Saposins A, B, C and D comprise a family of small, non-enzymatic lipid-transfer proteins that are essential for the activation of GSL catabolism; genetic defects in saposin function cause specific forms of lysosomal storage diseases. Each saposin shows functional specificity for the activation of certain catabolic reactions: saposin A (SapA) activates the hydrolysis of β-d-galactocerebroside to ceramide and galactose by the enzyme β-galactocerebrosidase (GALC; EC 3.2.1.46; Morimoto et al., 1989; Harzer et al., 1997). Whilst they share less than 35% sequence identity, they all adopt a common fold consisting of four amphipathic α-helices organized into two ‘fingers’. SapA is known to bind lipids and detergents in a pH-dependent manner; this is accompanied by a striking transition from a ‘closed’ to an ‘open’ conformation.

However, previous structures were determined at non-lysosomal pH. This work describes a 1.8 Å resolution X-ray crystal structure determined at the physiologically relevant lysosomal pH 4.8. In the absence of lipid or detergent at pH 4.8, SapA is observeed to adopt a conformation closely resembling the previously determined ‘closed’ conformation, showing that pH alone is not sufficient for the transition to the ‘open’ conformation. The asymmetric unit contains two molecules of SapA, both in the closed conformation, with the characteristic saposin fold. Analysis with PDBePISA suggests that the two molecules in the asymmetric unit form a crystallographic pseudodimer and not a stable quaternary complex. This is consistent with observations that SapA remains monomeric at low pH in the absence of detergent. The two chains observed in the asymmetric unit are almost identical, with a backbone r.m.s.d. of 0.46 Å after least-squares alignment. The largest difference was seen at Trp37, which was observed in a dual-occupancy conformation in chain B only, indicating that this side chain is mobile. Comparison of atomic B factors shows that the α3–α4 hinge region is more ordered in both chains of the pH 4.8 structure than in the pH 6.0 structure. There are no large-scale conformational rearrangements accompanying pH change, emphasizing the absolute necessity of lipids or detergents for transition to the open conformation. However, in combination with the structure of closed SapA at pH 6.0, this work reveals regions of conformational flexibility, and the crystal packing suggests a tendency to bury the negatively charged α3 helix at lysosomal pH.

>MGSLPCDICKDVVTAAGDMLKDNATEEEILVYLEKTCDWLPKPNMSASCKEIVDSYLPVILDIIKGEMSRPGEVCSALNLCESLQ[2x]> GSHMTETVPLILLVPKSRREDLEKAQLAERLRSQFFIDYGVRLPEVLLRDGEGLDDNSIVLLINEIRVEQFTVYFDLMRVVNYSDEVVSFGINPTIHQQGSSQYFWVTHEEGEKLRELGYVLRNALDELYHCLAVTLARNVNEYFGIQETKHMLDQLEAKFPDLLKEVLRHATVQRISEVLQRLLSERVSVRNMKLIMEALALWAPREKDVINLVEHIRGAMARYICHKFANGGELRAVMV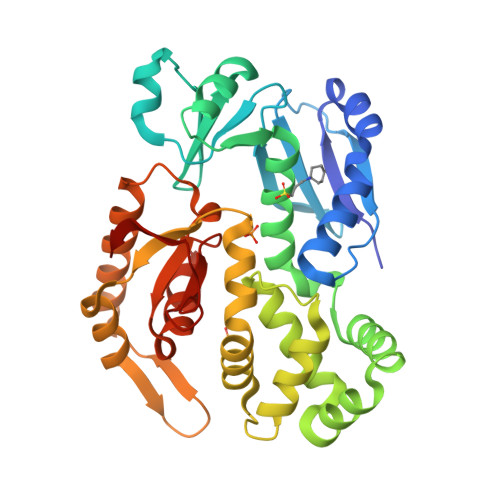SAEVEDVIRKGIRQTSGSTFLSLDPEASANLMDLITLKLDDLLIAHKDLVLLTSVDVRRFIKKMIEGRFPDLEVLSFGEIADSKSVNVIKTI>[4x]GGGGGPGELGKPVRLPKEMSDEMKKAVDDGWTKNAFNQYVSDLISVHRTLPDPRDAWCKDEARYLTNLPKTDVIICFHNEAWTVLLRTVHSVLDRSPEHLIGKIILVDDYSDMPHLKRQLEDYFAAYPKVQIIRGQKREGLIRARILGANHAKSPVLTYLDSHCECTEGWLEPLLDRIARNSTTVVCPVIDVISDETLEYHYRDSGGVNVGGFDWNLQFSWHPVPERERKRHNSTAEPVYSPTMAGGLFSIDREFFDRLGTYDSGFDIWGGENLELSFKTWMCGGTLEIVPCSHVGHIFRKRSPYKWRSGVNVLKKNSVRLAEVWMDEYSQYYYHRIGNDKGDWGDVSDRRKLRNDLKCKSFKWYLDNIYPELFIPGDSVAHGEIRNLGYGGRTCLDAPAGKKHQKKAVGTYPCHRQGGNQYWMLSKAGEIRRDDSCLDYAGKDVTLFGCHGGKGNQFWTYRENTKQLHHGTSGKCLAISESKDKLLMEECSASLSRQQWTLENYDSSKL

CG30463 is predicted to encode a ppGalNAcT/PGANT, which is an O-glycosyltransferase responsible for the post-translational addition of the sugar N-acetylgalactosamine (GalNAc) to proteins, a modification typically found on mucins and other secreted and membrane-bound proteins. ppGalNAcTs are type II membrane proteins that belong to the CAZy family GT2731. Interestingly, we found two distinct Drosophila cDNA clones emanating from the CG30463 gene, differing only in a ~30 amino acid region (the α subunit) of the lectin domain. Comparison of these clones to genomic sequence data revealed that they represent splice variants of exon 8. This splicing event generates an α subunit with a net positive charge (isoform A, containing exon 8A) or a net negative charge (isoform B, containing exon 8B). PGANT9A and PGANT9B adopt the canonical ppGalNAcT tertiary structure where a ~10 amino acid flexible linker connects the N-terminal catalytic domain to the C-terminal lectin domain.

PGANT9A crystallizes with 4 molecules in the asymmetric unit, and each molecule contains electron density in the active site consistent with a catalytic Mn2+ ion coordinated by the conserved active site residues Asp 301, His 303, and His 437, and 2 oxygens from the α and β phosphate of UDP. However, there is insufficient electron density to model in a peptide, and the partially ordered active site loop containing residues Arg 440 to Arg 448 is in a semi-closed conformation. In PGANT9A, Lys 542, Lys 543, Lys 546, and Lys 547 in the α subunit loop form a basic patch that extends towards the active site with the shortest distance of ~14 Å from Lys 542 to the nearest UDP phosphate. Arg 526, Arg 533, and Arg 556 form a distinct basic patch at the opposite end of the α subunit. The distribution of positively charged residues in the α subunit of PGANT9A creates a predominantly positively charged patch that extends the entire length of the lectin domain, and the proximity of the positively charged loop to the active site suggests that it dictates preferences for substrates that contain negatively charged residues, as the positively charged surface could form non-specific electrostatic interactions with the substrate to position it for catalysis. Likewise, positively charged substrates might be excluded from accessing the active site given the position of the positively charged loop. Thus, both enzymes have two distinct charged patches in their lectin domain formed by the α-subunit that results in preferences to recruit either negatively (PGANT9A) or positively (PGANT9B) charged substrates to the active site for catalysis. In PGANT9A and PGANT9B, the loop is closer to the active site than in the other ppGalNAcTs. To further interrogate this model, we redesigned the PTTTK peptide to replace all positively charged amino acids with negatively charged ones (PTTTE peptide; PTTTEPTTTEPTTTE).>GHMQMPGIENIPATLSHGGRFIQYNIFGNIFEVTAKYKPPIMPIGKGAYGIVCSAMNSETNESVAIKKIANAFDNKIDAKRTLREIKLLRHMDHENIVAIRDIIPPPLRNAFNDVYIAYELMDTDLHQIIRSNQALSEEHCQYFLYQILRGLKYIHSANVLHRDLKPSNLLLNANCDLKICDFGLARVTSESDFMTEYVVTRWYRAPELLLNSSDYTAAIDVWSVGCIFMELMDRKPLFPGRDHVHQLRLLMELIGTPSEEELEFLNENAKRYIRQLPPYPRQSITDKFPTVHPLAIDLIEKMLTFDPRRRITVLDALAHPYLNSLHDISDEPECTIPFNFDFENHALSEEQMKELIYREALAFNPEYQQ[2x]

Mitogen-activated protein kinase (MAPK) cascades, which are composed of MAPK kinase kinase, MAPK kinase and MAPK (called MAPKKK, MAPKK, and MAPK), are highly conserved signalling modules in eukaryotic organisms. MAPKKs are dual-specificity kinases that activate MAPKs by phosphorylating the threonine and tyrosine residues in their conserved TXY motif. Arabidopsis MPK3 and MPK6 were shown to be activated by multiple MKKs, including MKK2, MKK3, MKK4, MKK5, MKK7, and MKK9, and are involved in the regulation of biotic and abiotic stress responses and growth and development processes16171819202122232425. Activated MPK6 phosphorylates a variety of substrates, including enzymes, transcription factors, and cellular structural proteins21262728293031.

Here, we present the crystal structure of the unphosphorylated Arabidopsis MPK6 at 3.0 Å resolution. MPK6Δ1–28, a mutant with the shortest amino acid residue deletion in our experiment (with 1–28 amino acid residues deleted), was shown to be phosphorylated and activated by MKK5DD to a similar level as MPK6. The present model of MPK6 includes amino acid residues 29 to 395. The MPK6 crystals contain two protein chains in the asymmetric unit. Amino acid residues 70–75 (part of the glycine-rich loop), 213–214 (part of the phosphorylation lip), and 366–374 (part of the L16 loop) in chain A and amino acid residues 215–224 (phosphorylation lip) and 285–287 (part of the MAPK insert) in chain B were not resolved in the electron density maps. The N-lobe (residues 32–147 and 360–394) contains eight β-strands (β1 to β5, β0L0, β1L0, and β2L0) and two α-helices (αC and αL16), whereas the C-lobe (residues 149–359) consists of six α-helices (αD to αI) and three short β-strands (β6-β8). The structure reveals that although MPK6 is topologically similar to the non-plant MAPKs, the structures of the glycine-rich loop, MAPK insert, and L16 loop in MPK6 are saliently different from those of MAPKs. Compared with inactive ERK2 and p38α, the glycine-rich loop in MPK6 folds down onto the ATP binding pocket and is closer to the phosphorylation lip. First, the MKI of MPK6 does not form α1L14 (285–289) but only contains α2L14 (residues 293–301) and a 3/10 helix. Compared to ERK2 and p38, the structure of the MPK6 L16 loop does not fit in the groove, due to hindrance from the side chains of Phe364, Phe366, and Phe368 in L16.>[2x]MSGTEDERRELEKVARKAIEAAREGNTDEVREQLQRALEIARESGSEEAFKLALEVVRRVAEVAARAGNVEAVKEALRVALEIVKEAMELIKDPEAIVRLALEAVRVVAEVAARAGAVEAVKVALRVALEIAKIAGTEEAVRLALEVVKRVSDIAKKAGNEDAVKEAEEVRKKIEEESGGSGMEEARKELTREMIEVLREIEEGFKERFE

We set out to design proteins that can switch between two well-defined and fully structured conformations. We reasoned that these goals could be collectively achieved with a “hinge”-like design in which two rigid domains move relative to each other while remaining individually folded. The hinge amplifies small local structural and chemical changes to achieve large global changes while the chemical environment for most residues remains similar throughout the conformational change, avoiding the need for global unfolding. Designing one of the resulting conformations to bind to a target effector couples the conformational equilibrium with target binding.

To generate a second conformation, a copy of the parent protein is rotated around a “pivot helix” and a new backbone conformation is then created by combining the first half of the original protein (domain 1), the second half of the copy (domain 2), and either the helix following the pivot helix from the original protein or the helix preceding the pivot helix from the rotated copy (“peptide”). Using a combination of Rosetta two-state design (see methods section for details) and proteinMPNN(27) with linked residue identities, a single amino acid sequence is generated that is compatible with the state X hinge as well as with the state Y hinge-peptide complex. We solved crystal structures for two designs, cs207 and cs074. For design cs207, crystals were obtained from two separate crystallization screens: one screen for the hinge alone, and one screen for the hinge in complex with the target peptide. In the absence of peptide the experimental structure agrees well with the state X design model, and the structure of the hinge-peptide complex agrees well with the state Y design model. The crystal structures of hinge cs207 in both designed states demonstrate the accuracy with which two very different conformational states of the same protein can now be designed.>[2x]SNAMPLPKSLKYGDTIGIYSPSSPVTYTSPKRFERAKSYLLQKGFHILEGSLTGRYDYYRSGSIQERAKELNALIRNPNVSCIMSTIGGMNSNSLLPYIDYDAFQNNPKIMIGYSDATALLLGIYAKTGIPTFYGPALVP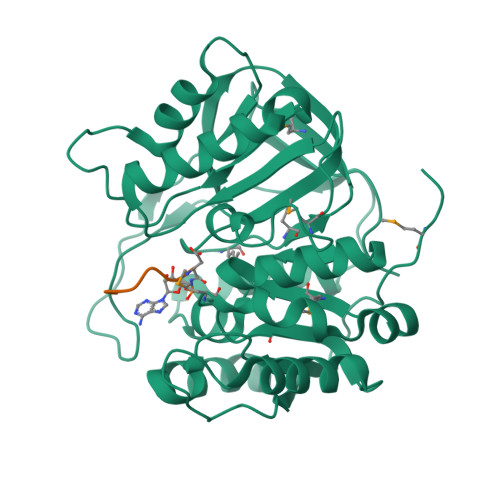SFGEFEPFVDDTYKYFLETLLHDQALPYNIKQPLFWSDEFINWEEKTKEKELRPNNWISVTNGQATGRVIGGNLNTIQGIWGSPYMPCIQEGDILFIEDSSKDAATIERSFSFLKINGVFDKVSGIILGKHEQFDDCGTNRKPYEILLEVLQNQRIPLLADFDCCHTHPMITMPIGVQVKMDATNKTIHILEKWKI;>[2x]MRTGNAN> MGVVEEAHNVKVIGSGEATIVLGHGFGTDQSVWKHLVPHLVDDYRVVIYDNMGAGTTNPDYFDFDRYSNLEGYSFDLIAILEDLKIESCIFVGHCVSAMIGVLASLNRPDLFSKIVMISASPRYVNDVDYQGGFEQEDLNQLFEAIRSNYKAWCLGFAPLAVGGDMDSIAVQEFSRTLFNMRPDIA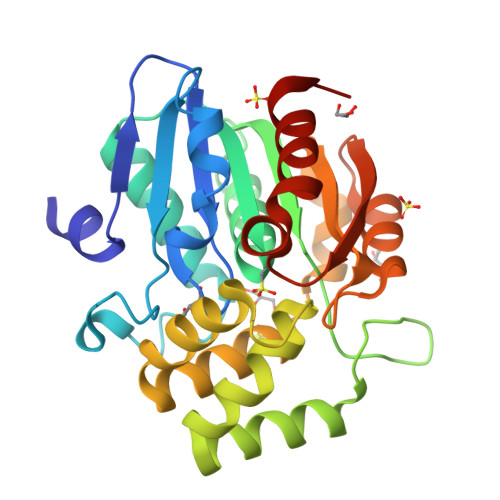LSVGQTIFQSDMRQILPFVTVPCHILQSVKDLAVPVVVSEYLHANLGCESVVEVIPSDGHLPQLSSPDSVIPVILRHIRNDIAM>MQIGRVRGTVVSSQKEPSMVGVKFLLLQLIDEAGQPLPQYEVAADGVGAGLDEWVLFSRGSAARQVAGSEKRPVDAVVIGIIDTVSVDNRPLYSKKDQYRGSHHHHHH[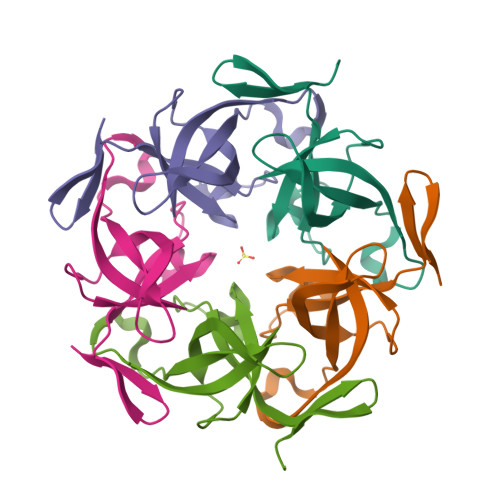5x]> GSHMGIKQKSYQPSIIIAGPQNSGKTSLLTLLTTDSVRPTVVSQEPLSAADYDGSGVTLVDF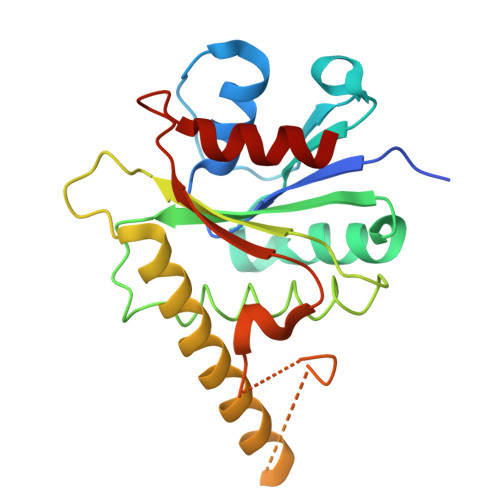PGHVKLRYKLSDYLKTRAKFVKGLIFMVDSTVDPKKLTTTAEFLVDILSITESSCENGIDILIACNKSELFTARPPSKIKDALESEIQKVIERRKKSLNEVERKINEEDYAENTLDVLQSTDGFKFANLEASVVAFEGSINKRKISQWREWIDEKL N-(3-tert-butyl-1-phenyl-1H-pyrazol-5-yl)-2-{[1-(4-hydroxyphenyl)-1H-tetrazol-5-yl]sulfanyl}acetamide 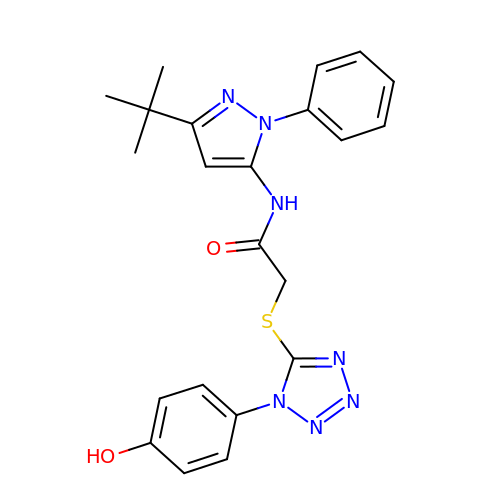| C22 H23 N7 O2 S | MLPOPBODRFYIRV-UHFFFAOYSA-N>[2x]GSHMLDMTRIILPGKTIGIIGGGQLGRMMALAAKEMGYKIAVLDPTKNSPCAQVADIEIVASYDDLKAIQHLAEISDVVTYEFENIDYRCLQWLEKHAYLPQGSQLLSKTQNRFTEKNAIEKAGLPVATYRLVQNQEQLTEAIAELSYPSVLKTTTGGYDGKGQVVLRSEADVDEARKLANAAECILEKWVPFEKEVSVIVIRSVSGETKVFPVAENIHVNNILHESIVPAR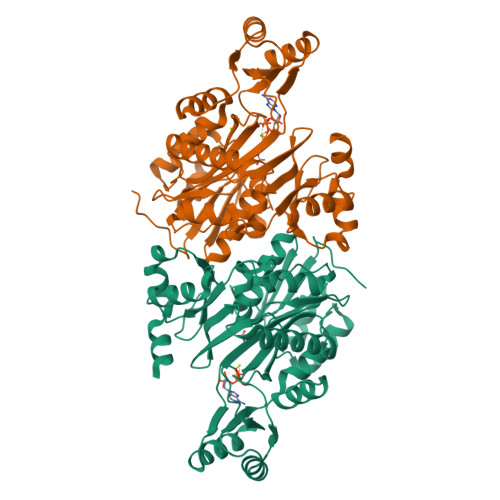ITEELSQKAIAYAKVLADELELVGTLAVEMFATADGEIYINELAPRPHNSGHYTQDACETSQFGQHIRAICNLPLGETNLLKPVVMVNILGEHIEGVLRQVNRLTGCYLHLYGKEEAKAQRKMGHVNILNDNIEVALEKAKSLHIWDHQEQLLEG> GLGGLERFCSPGKGRGLRALQPFQVGDLLFSCPAYAYVLTVNERGNHCEYCFTRKEGLSKCGRCKQAFYCNVECQKEDWPMHKLECSPMVVFGENWNPSETVRLTARILAKQKIHPERTPSEKLLAVKEFESHLDKLDNEKKDLIQSDIAALHHFYSKHLEFPDNDSLVVLFAQVNCNGFTIEDEELSHLGSAIFPDVALMNHSCCPNVIVTYKGTLAEVRAVQEIKPGEEVFTSYIDLLYPTEDRNDRLRDSYFFTCECQECTTKDKDKAKVEIRKLSDPPKAEAIRDMVRYARNVIEEFRRAKHYKSPSELLEICELSQEKMSSVF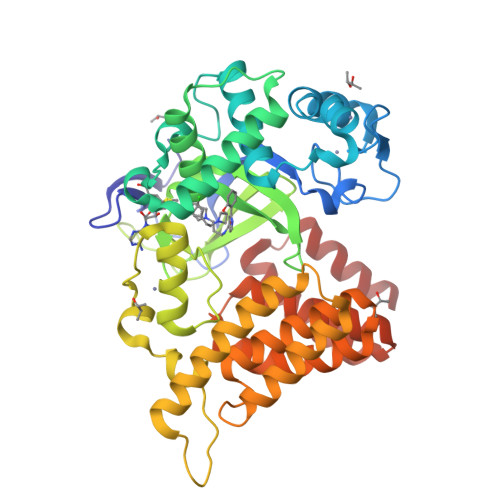EDSNVYMLHMMYQAMGVCLYMQDWEGALQYGQKIIKPYSKHYPLYSLNVASMWLKLGRLYMGLEHKAAGEKALKKAIAIMEVAHGKDHPYISEIKQEIESH> GHMSLSKKRKLESGDSGGAGAGGEGAEEENGGEQEAAPPRPRRTKSERDQLYYECYSDVSVHEEMIADQVRTEAYRLGILKNWAALRGKTVLDVGAGTGILSIFCAQAGARRVYAVEASAIWQQAREVVRLNGLEDRVHVLPGPVETVELPERVDAIVSEWMGYGLLHESMLSSVLHARTKWLKEGGL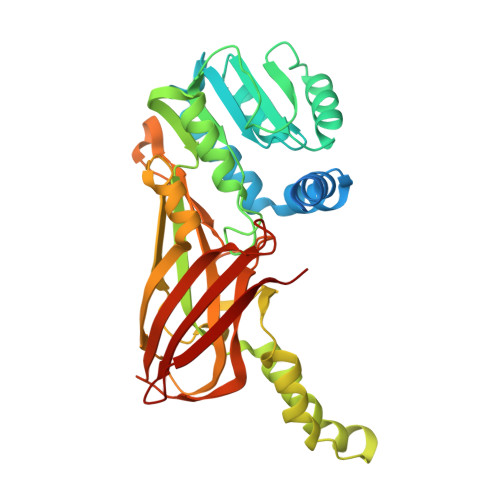LLPASAELFVAPISDQMLEWRLGFWSQVKQHYGVDMSCMESFATRCLMGHSEIVVQDLSGEDVLARPQRFAQLELARAGLEQELEAGVGGRFRCSCYGSAPLHGFAVWFQVTFPGGDSEKPLVLSTSPLHPATHWKQALLYLNEPVPVEQDTDISGEITLLPSPDNPRRLRILLRYKVGDHEEKTKDFAMED>[2x]GPGSAMKAPELKEKLEESEKLIKELTVTWEEKLRKTEAIAQERQRQLESMGISLETSGIKVGDDKCYLVNLNADPALNELLVYYLKDHTRVGADTSQDIQLFG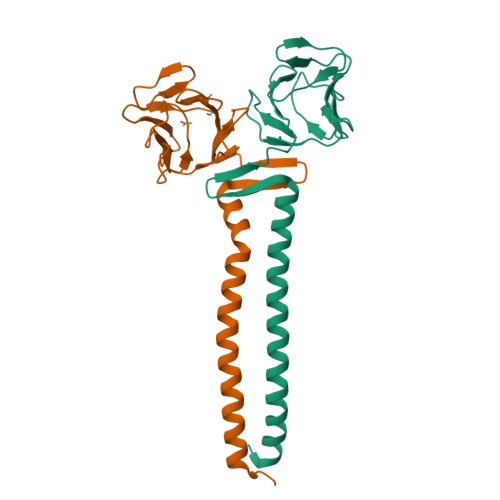IGIQPEHCEIDIAADGDITLTPKENARSCVNGTLVCSTTQLWHGDRILWGNNHFFRINLPKRKRRDWLKDF> MMRVNFDTLYSNYPSSDPSHPNYLSQRDLFTEIGWESFIGNPNYHNTCAIRVSIAFVKSGINIVPSSHRIQKGPY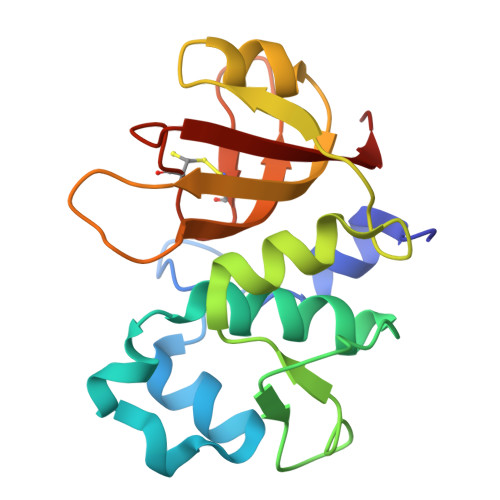AGKGIEVNMRRLATLMKRTSYLGEPDPYTPATARNGIGARNGVVAFNNIPGYTGGGHIDLVRGGSEATQCASACYYNSETIWFWPLQAS> APLADYKDDDDKLAGTPSVDHGFLVTRHSQTIDDPQCPSGTKILYHGYSLLYVQGNERAHGQDLGTAGSCLRKFSTMPFLFCNINNVCNFASRNDYSYWLSTPEPMPMSMAPITGENIRPFISRCAVCEAPAMVMAVHSQTIQIPPCPSGWSSLWIGYSFVMHTSAGAEGSGQALASPGSCLEEFRSAPFIECHGRGTCNYYANAYSFWLATIERSEMFKKPTPSTLKAGELRTHVSRCQVCMGTGYLLVKHSQTDQEPMCPVGMNKLWSGYSLLYFEGQEKAHNQDLGLAGSCLARFSTMPFLYCNPGDVCYYASRNDKSYWLSTTAPLPMMPVAEDEIKPYISRCSVCEAPAIAIAVHSQDVSIPHCPAGWRSLWIGYSFLMHTAAGDEGGGQSLVSPGSCLEDFRATPFIECNGGRGTCHYYANKYSFWLTTIPEQSFQGSPSADTLKAGLIRTHISRCQVCMAPGFLVTRHSQTIDDPQCPSGTKILYHGYSLLYVQGNERAHGQDLGTAGSCLRKFSTMPFLFCNINNVCNFASRNDYSYWLS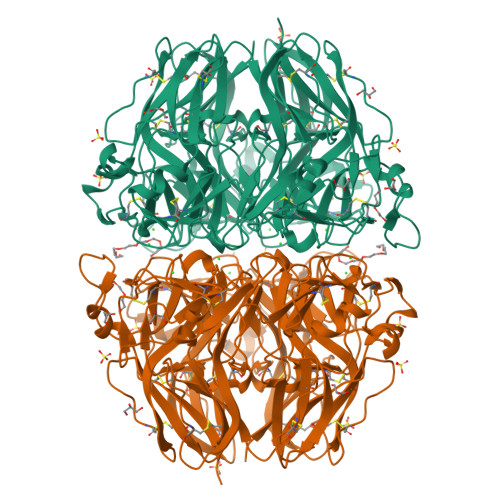TPEPMPMSMAPITGENIRPFISRCAVCEAPAMVMAVHSQTIQIPPCPSGWSSLWIGYSFVMHTSAGAEGSGQALASPGSCLEEFRSAPFIECHGRGTCNYYANAYSFWLATIERSEMFKKPTPSTLKAGELRTHVSRCQVCMRRT> QGHMVSAEGRNRKAVLCQRCGSRVLQPGTALFSR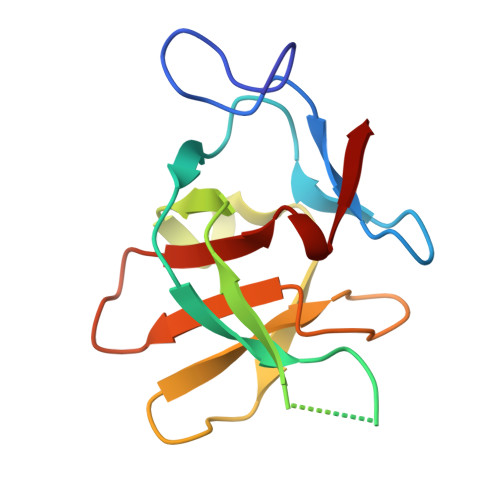RQLFLPSMRKKPALSDGSNPDGDLLQEHWLVEDMFIFENVGFTKDVGNIKFLVCADCEIGPIGWHCLDDKNSFYVALERVSHE>SSKLQALFAHPLYNVPEEPPLLGAEDSLLASQEALRYYRRKVARWNRRHKMYREQMNLTSLDPPLQLRLEASWVQFHLGINRHGLYSRSSPVVSKLLQDMRHFPTISADYSQDEKALLGACDCTQIVKPSGVHLKLVLRFSDFGKAMFKPMRQQRDEETPVDFFYFIDFQRHNAEIAAFHLDRILDFRRVPPTVGRIVNVTKEILEVTKNEILQSVFFVSPASNVCFFAKCPYMCKTEYAVCGKPHLLEGSLSAFLPSLNLAPRLSVPNPWIRSYTLAGKEEWEVNPLYCDTVKQIYPYNNSQRLLNVIDMAIFDFLIGNMDRHHYEMFTKFGDDGFLIHLDNARGFGRHSHDEISILSPLSQCCMIKKKTLLHLQLLAQA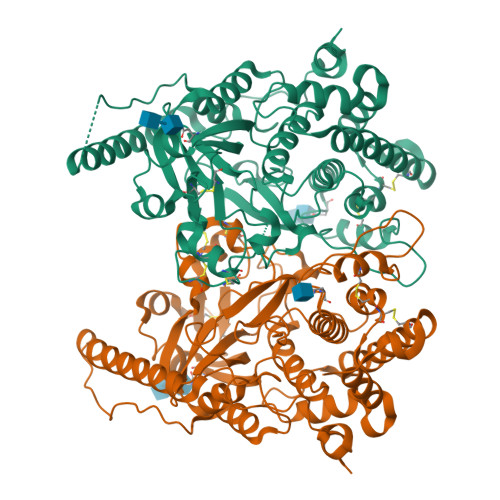DYRLSDVMRESLLEDQLSPVLTEPHLLALDRRLQTILRTVEGCIVAHGQQSVIVDGP[2x]>ALANTFLVKEDSKNVTAYTPFATPITDSKSDLVSLAQLDSSYQIADQTIHNTNLFVLFKSRDVKVKYESSGSNNISFDSTSQGEKPSYVVEFTNSTNIGIKWTMVKKYQLDVPNVSSDMNQVLKNLILEQPLTKYTLNSSLAKEKGKTQREVHLGSGQANQWTSQRNQHDLNNNPSPNASTGFKLTTGNAYRKLSESWPIYEPIDGTKQGKGKDSSGWSSTEENEAKNDAPSVSGGGSSSGTFNKYLNTKQALESIGILFDDQTPRNVITQLYYASTSKLAVTNNHIVVMGNSFLPSMWYWVVERSAQENASNKPTWFANTNLDWGEDKQKQFVENQLGYKETTSTNSHNFHSKSFTQPAYLISGIDSVNDQIIFSGFKAGSVGYDSSSSSSSSSSSSTKDQALAWSTTTSLDSKTGYKDLVTNDTGLNGPINGSFSIQDTFSFVVPYSGNHTNNGTTGPIKTAYPVKKDQKSTVKINSLINATPLNSYGDEGIGVFDALGLNYNFKSNQERLPSRTDQIFVYGIVSPNELRSAKSSADSTGSDTKVNWSNTQSRYLPVPYNYSEGIIDADGFKRPENRGASVTTFSGLKSIAPDGFANSIANFSVGLKAGIDPNPVMSGKKANYGAVVLTRGGVVRLNFNPGNDSLLSTTDNNIAPISFSFTPFTAAESAVDLTTFKEVTYNQESGLWSYIFDSSLKPSHDGKQTPVTDNMGFSVITVSRTGIELNQDQATTTLDVAPSALAVQSGIQSTTQTLTGVLPLSEEFSAVIAKDSDQNKIDIYKNNNGLFEIDTQLSNHHHHHH[4x];>GVITGVGGYFLFNQNKQRSSVSNFAYQPKQLSVKHQQAVDETLTPWTWNNNNFSSLKITGENPGSFGLVRSQNDNLNISSVTKNSSDDNLKYLNAVEKYLDGQQNFAIRRYDNNGRALYDINLAKMENPSTVQRGLNGEPIFDPFKGFGLTGNAPTDWNEIKGKVPVEVVQSPHSPNLYFVLLVPKVALEYHNLNNQVVKESLEVKATQSSFNPTQRLQKDSPVKDSSKQGEKLSETTASSMSSGMATSTRAKALKVEVERGSQSDSLLKNDFAKKPLKHKNSSGEVKLEAEKEFTEAWKPLLTTDQIAREKGMGATVVSFYDAPYSENHTAFGLVDHIDPKKMVENYPPSWKTPKWNHHGIWDYNARNLLLQTTGFFNPRRHPEWFDEGQAKADNTSPGFKVGDTDHKKDGFKKNSSSPIALPFEAYFANIGNMVAIGNSVFIFGGNGHATKMFTTNPLSIGVFRIKYTDNFSKSSVTGWPYAVLFGGLINPQTNGLKDLPLGTNRWFEYVPRMAVSGVKWVGNQLVLAGTLTMGDTATVPRLKYDQLEKHLNLVAQGQGLLREDLQIFTPYGWANRPDIPVGAWLQDEMGSKFGPHYFLNNPDIQDNVNNDTVEALISSYKNTDKLKHVYPYRYSGLYAWQLFNWSNKLTNTPLSANFVNENSYAPNSLFAAILNEDLLTGLSDKIFYGKENEFAENEADRFNQLLSLNPNPNTNWARYLNVVQRFTTGPNLDSSTFDQFLDFLPWIGNGKPFSNSPSPSTSASSSTPLPTFSNINVGVKSMITQHLNKENTRWVFIPNFSPDIWTGAGYRVQSANQKNGIPFEQVKPSNNSTPFDPNSDDNKVTPSGGSSKPTTYPALPNSISPTSDWINALTFTNKNNPQRNQLLLRSLLGTIPVLINKSGDSNDQFNKDSEQKWDKTETNEGNLPGFGEVNGLYNAALLHTYGFFGTNTNSTDPKIGFKADSSSSSSSTLVGSGLNWTSQDVGNLVVINDTSFGFQLGGWFITFTDFIRPRTGYLGITLSSLQDQTIIWADQPWTSFKGSYLDSDGTPKSLWDPTALKSLPNSSTTYDTNPTLSPSFQLYQPNKVKAYQTTNTYNKLIEPVDATSAATNMTSLLKLLTTKNIKAKLGKGTASSQGNNNGGGVSQTINTITTTGNISEGLKEETSIQAETLKKFFDSKQNNKSEIGIGDSTFTKMDGKLTGVVSTPLVNLINGQGATSDSDTEKISFKPGNQIDFNRLFTLPVTELFDPNTMFVYDQYVPLLVNLPSGFDQASIRLKVISYSVENQTLGVRLEFKDPQTQQFIPVLNASSTGPQTVFQPFNQWAHHHHHH[4x]

The human pathogen Mycoplasma genitalium, a member of the pneumoniae cluster of mycoplasmas, binds to eukaryotic cells by means of its adhesion complex, the Nap. This complex is formed by two heterodimers, each consisting of proteins P110 and P1401–6. In addition to their roles in cytadherence and motility, P110 and P140 are immunodominant proteins and constitute the main target of host antibodies during infection. Here, we address the structure and mechanism of the Nap adhesion complex and reveal an intricate interplay between P110 and P140.

Crystals were obtained from the extracellular region of P140 (residues 23–1351), both alone and in complex with the N-terminal domain of P110 (P110N: residues 23–827). The structure of P140, for which there are no molecular models or experimental phases available, was determined by density modification techniques, starting with a mask derived from the sub-tomogram-averaged map of the whole Nap obtained by cryo-electron tomography (cryo-ET). With four heterodimers in the asymmetric unit, the P140–P110N crystals were refined at 2.65 Å resolution to a final model with agreement R and Rfree factors of 18.7 and 22.4, respectively. The binding site for the sialylated oligosaccharides, identified in the structure of P1106, is located at the interface between P140 and P110 in the crystal structure of the P140–P110N complex. Interaction of the two subunits changes the position of the sialic binding β-hairpin while the interfering loop (P140 residues 807–827) inserts into the binding pocket of P110N, sterically interfering with the binding of oligosaccharides to the complex. In agreement with this, surface plasmon resonance analysis shows that, in solution, sialylated compounds 3SL and 6SL (neuraminic acid forming an α2–3 or an α2–6 linkage to a lactose monosaccharide, respectively), which bind to P110 alone, do not bind either to P140 alone or to P140–P110 complexes. The structure of the P140–P110N complex suggests that P110 residues Gln460–Asp461, from the binding β-hairpin, and Arg600, close to the receptor-binding site, play an important role in the interaction with P140. P110 variants carrying an R600A substitution or the triple substitution RQD (R600A, Q460A, and D461A) were introduced by transposon delivery into an M. genitalium P110 null mutant. Strains expressing the P110-RQD variant protein, which was barely detectable, showed a null binding capacity phenotype. The variant protein P110-R600A was well expressed, but the strain presented no capacity for adherence and characterization of cell motility was not feasible. The “closed” conformation corresponds to a state in which the tight interaction of the extracellular regions of P140 and P110 occlude the cell receptor-binding site.> AKTHSVETPYGSVTFTVYGTPYPYRPAILTYHDVGLNYKSCFQPLFQFEDMQEIIQNFVRVHVDAPGMEEGAPVFPLGYQYPSLDQLADMIPCVLQYLNFSTIIGVGVGAGAYILARYALNHPDTVEGLVLINIDPNAKGWMDWAAHKLTGLTSSIPEMILGHLFSQEELSGNSELIQKYRNI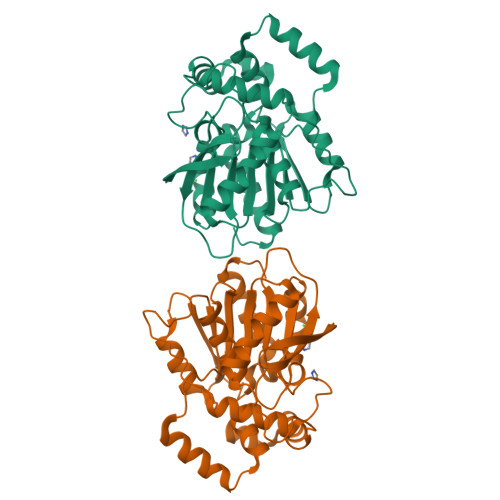ITHAPNLDNIELYWNSYNNRRDLNFERGGDITLRCPVMLVVGDQAPHEDAVVECNSKLDPTQTSFLKMADSGGQPQLTQPGKLTEAFKYFLQGMGYMA>[7x]MSIPVTEFRQFSEQQPAFRVLKPWWDVFTDYLSVAMLMIGVFGCTLQVMQDKIICLPKRVQPAQNHSSLSNVSQAVASTTPLPPPKPSPANPITVEMKGLKTDLDLQQYSFINQMCYERALHWYAKYFPYLVLIHTLVFMLCSNFWFKFPGSSSKIEHFISILGKCFDSPWTTRALSEVSGEDSEEKDNRKNNMNRSNTIQSGPEGSLVNSQSLKSIPEKFVVDKSTAGALDKKEGEQAKALFEKVKKFRLHVEEGDILYAMYVRQTVLKVIKFLIIIAYNSALVSKVQFTVDCNVDIQDMTGYKNFSCNHTMAHLFSKLSFCYLCFVSIYGLTCLYTLYWLFYRSLREYSFEYVRQETGIDDIPDVKNDFAFMLHMIDQYDPLYSKRFALFLSEVSE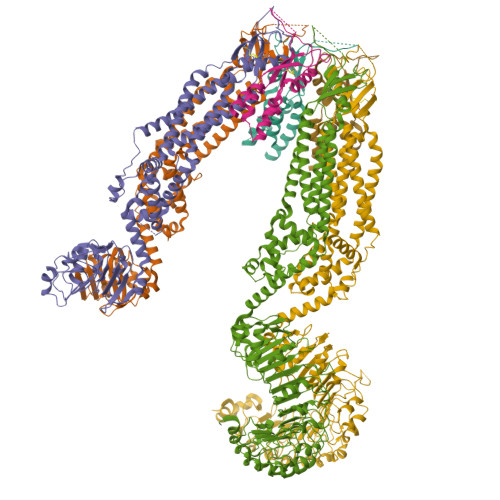NKLKQLNLNNEWTPDKLRQKLQTNAHNRLELPLIMLSGLPDTVFEITELQSLKLEIIKNVMIPATIAQLDNLQELSLHQCSVKIHSAALSFLKENLKVLSVKFDDMRELPPWMYGLRNLEELYLVGSLSHDISRNVTLESLRDLKSLKILSIKSNVSKIPQAVVDVSSHLQKMCIHNDGTKLVMLNNLKKMTNLTELELVHCDLERIPHAVFSLLSLQELDLKENNLKSIEEIVSFQHLRKLTVLKLWHNSITYIPEHIKKLTSLERLSFSHNKIEVLPSHLFLCNKIRYLDLSYNDIRFIPPEIGVLQSLQYFSITCNKVESLPDELYFCKKLKTLKIGKNSLSVLSPKIGNLLFLSYLDVKGNHFEILPPELGDCRALKRAGLVVEDALFETLPSDVREQMKADALEVLFQ Human cellular retinol binding protein II (hCRBPII) was used as a protein engineering platform to rationally regulate absorptive and emissive properties of a covalently bound fluorogenic dye. We demonstrate the binding of a thio-dapoxyl analog via formation of a protonated imine between an active site lysine residue and the chromophore’s aldehyde. Previously, we showed the utility of human cellular retinol-binding protein II (hCRBPII) mutants as a fluorophoric tag, wherein an active site lysine residue (Q108K) reacts with synthetic aldehydic chromophores, giving rise to the formation of either an imine (Schiff base, SB) or an iminium (protonated SB, PSB). Q108K functions as the active-site lysine and forms a Schiff base with the aldehyde, whereas the K40L mutation is assumed to eliminate interactions between Q108K and Lys40, an interaction that could otherwise impede imine formation, and is also required to promote Schiff base protonation.

Introduction of acidic residues near the iminium should localize the positive charge on the iminium, resulting in a blue-shift of the absorption/emission of the protein/TD-1V complex. Our prior experience with these proteins also informed our decision to maintain the K40L mutant for stability concerns, and thus we pivoted our strategy by incorporating acidic residues into the previously red-shifted template M14. Subsequently, we mutated Leu117 to both Asp and Glu, resulting in a distinct, blue-shifted iminium (M22–M23). Nonetheless, we did observe a discernible pattern in the quantum yields of mutants featuring acidic residues proximal to the iminium moiety. Interestingly, these mutants exhibited higher quantum yields, most greater than 30%. We attribute this to the propensity for salt-bridge formation between acidic residues and the iminium, which putatively would lead to increased rigidity of the bound chromophore, and thus reduced vibrational freedom, which in turn would reduce nonradiative relaxation pathways. Additionally, it is expressed solely in its monomeric form. Importantly, there was no apparent background fluorescence in the red channel, signifying that TD-1V specifically labels the intended lysine residue without reacting with off-target amines.

>[2x]TRDQNGTWEMESNENFEGWMKALDIDFATRKIAVRLTQTLVIDQDGDNFKVKSTSTFWNYDVDFTVGVEFDEYTKSLDNRHVKALVTWEGDVLVCVQKGEKENRGWKKWIEGDKLYEELTCGDQVCRQVFKKK Encapsulins are protein nanocompartments that house various cargo enzymes, including a family of decameric ferritin-like proteins. Cargo enzymes are directed inside the encapsulin nanocompartment by a terminal localization sequence (LS) that binds to the interior face of the encapsulin. EncFtn oxidizes iron in a similar manner to other ferritins, but due to its open structure, it must be associated with an encapsulin nanocage to act as an iron store. Together, the encapsulin EncFtn (Enc:EncFtn) complex can perform both the oxidation and storage functions of classical ferritins. Here, we investigate the structure of the Enc:EncFtn nanocompartment from the halophilic bacterium Haliangium ochraceum to gain a better understanding of the arrangement and stoichiometry of the complex.

To capture the extreme open and closed conformations of the fivefold pores, we performed symmetry expansion on the I1 particle set in Relion3.1, followed by masked 3D classification without alignment centered on the vertex. The closed conformation has a fivefold pore diameter of 5 Å, while the equivalent diameter of the open conformation is 15 Å. The closed conformation of the fivefold pore is consistent with observations from the crystal structure of the T. maritima encapsulin and high-resolution cryo-EM structures of other encapsulins. To understand the structural changes taking place in the transition between these conformations, an atomic model of the encapsulin protein was refined against both maps. In addition, our focused refinements of the pentameric subunits allowed us to build and sequence the 117GSLGIGSLR125 peptide from the EncFtn protein. This region of the LS forms a network of hydrophobic interactions with the inner face of the P-domain of a single encapsulin monomer, with further stabilization by several water-mediated backbone contacts. The core GxLGIxxL motif found in this region of the LS is conserved between the H. ochraceum EncFtn and other proteins in the family and is observed in the crystal structure of the T. maritima encapsulin.

>[5x]MSSEQLHEPAELLSEETKNMHRALVTLIEELEAVDWYQQRADACSEPGLHDVLIHNKNEEVEHAMMTLEWIRRRSPVFDAHMRTYLFTERPILELEEEDTGSSSSVAASPTSAPSHGSLGIGSLRQEGKED;>[5x]MDLLKRHLAPIVPDAWSAIDEEAKEIFQGHLAGRKLVDFRGPFGWEYAAVNTGELRPIDDTPEDVDMKLRQVQPLAEVRVPFTLDVTELDSVARGATNPDLDDVARAAERMVEAEDSAIFHGWAQAGIKGIVDSTPHEALAVASVSDFPRAVLSAADTLRKAGVTGPYALVLGPKAYDDLFAATQDGYPVAKQVQRLVVDGPLVRANALAGALVMSMRGGDYELTVGQDLSIGYAFHDRSKVELFVAESFTFRVLEPGAAVHLRYA>[2x]TYTTRQIGAKNTLEYKVYIEKDGKPVSAFHDIPLYADKENN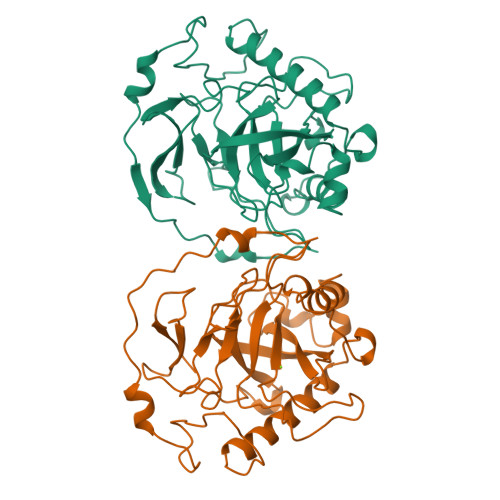IFNMVVEIPRWTNAKLEITKEETLNPIIQDTKKGKLRFVRNCFPHHGYIHNYGAFPQTWEDPNVSHPETKAVGDNDPIDVLEIGETIAYTGQVKQVKALGIMALLDEGETDWKVIAIDINDPLAPKLNDIEDVEKYFPGLLRATNEWFRIYKIPDGKPENQFAFSGEAKNKKYALDIIKETHDSWKQLIAGKSSDSKGIDLTNVTLPDTPTYSKAASDAIPPASLKADAPIDKSIDKWFF>[2x]GPLGSPEFP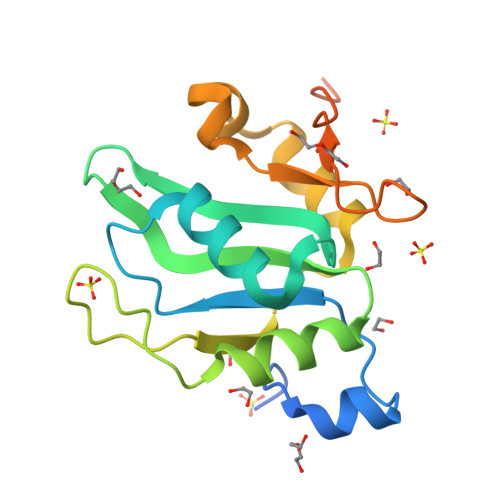GSDRNSVDYAQIASGIDTRTTVMIKNIPNKFTQQMLRDYIDVTNKGTYDFLYLRIDFVNKCNVGYAFINFIEPQSIITFGKARVGTQWNVFHSEKICDISYANIQGKDRLIEKFRNSCVMDENPAYRPKIFVSHGPNRGMEEPFPAPNNARRKLRSIASAQQIGLFPPTASKC alpha-D-ribofuranose | C5 H10 O5 | 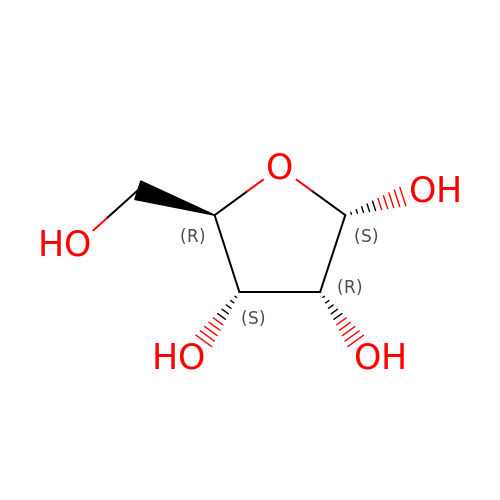HMFHBZSHGGEWLO-AIHAYLRMSA-N>MADTNRTDAAALIQEAYSDVFLDSVSETAKVIGTFPVYNMGTKTTNLPVLSTFPHAKWVGESATAPEGVKPTAKATWANK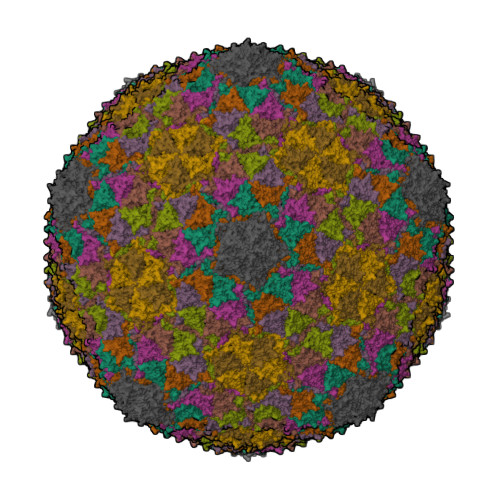TLVAEELAVILPIHENVLADATEDLLAELARMGGASIGRALDAAVLFGHQKPVTWASKSLFESADDAGQVVAVGNSNGVEGDDISGSILQAAEMVADVYDPSHLLGYSGLRYRLANQRDANGQPLFQPYMQGTPGSDGMVHGLNTVFFSGNVDDGSNGDAPVWDRDVASAIVVDRSRVVIGVRQDITVKYLDQATVGGINLAERDMVALRFCGRFAYALGDNIAQGRVAAENSPVAVITPYAGS[9x]>[4x]GSHMTTIILDCDPGHDDAMAILLALGNPNIDLLGVTTVG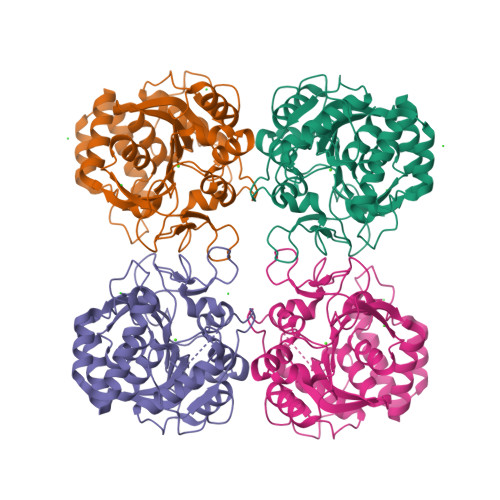GNQSLEKVTYNARATLEMAHATNIPVHAGCDRPMIRPLEVAAAVHGETGLDGVTLPEPTRPLDEGHAVNWIIDTIMSHEPGTITLVPTGPLTNIAMAVRLEPRIVSRVKEVVLMGGGYHVGNWSAVAEFNIKVDPEAAHVVFNEDWPITMVGLDLTHQALCTPEVQARIDAIGTPLSAFASGLMDFFRKAYKNNQDFIDPPVHDPCTVAYLIDHSVVQTRRCPVDVEIKGDLTLGMTVADLRGPEPSADKCHTQVATKLDFNKFWDLIIDALKELK(2S)-N-(3-chloro-2-methylphenyl)oxolane-2-carboxamide | C12 H14 Cl 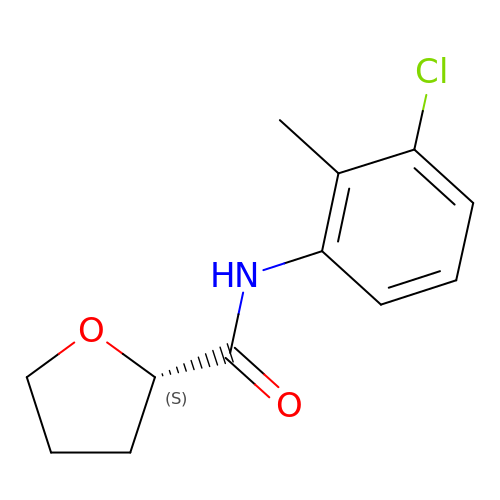N O2 | BKWNJEPRFSSIFE-NSHDSACASA-N>MGSSHHHHHHSSGLVPRGSHMSGSGSGSGTALTPSYLKDDDGRSLILRGFNTASSAKSAPDGMPQFTEADLAREYADMGTNFVRFLISWRSVEPAPGVYDQQYLDRVEDRVGWYAERGYKVMLDMHQDVYSGAITPEGNSGNGAGAIGNGAPAWATYMDGLPVEPQPRWELYYIQPGVMRAFDNFWNTTGKHPELVEHYAKAWRAVADRFADNDAVVAYDLMNEPFGGSLQGPAFEAGPLAAMYQRTTDAIRQVDQDTWVCVAPQAIGVNQGLPSGLTKIDDPRAGQQRIAYCPHLYPLPLDIGDGHEGLARTLTDVTIDAWRANTAHTARVLGDVPIILGEFGLDTTLP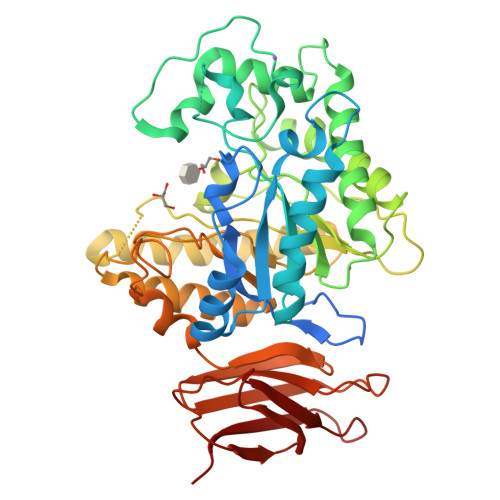GARDYIERVYGTAREMGAGVSYWSSDPGPWGPYLPDGTQTLLVDTLNKPYPRAVAGTPTEWSSTSDRLQLTIEPDAAITAPTEIYLPEAGFPGDVHVEGADVVGWDRQSRLLTVRTPADSGNVTVTVTPAA[2x]>[7x]GGVLVAQDYRAGSFIELLRNRMALAGVGVRILQGLTGNVDIPKRTGASTMYFVDEDVDVTESDGAFGLVGMTPHTAGVATAITRRMMQQGSPDIEALVRDDLLTSLTLGLDKTALVGHSSPSAPNGVRDLVIGDALPFTGPFATFEELVDLETAVASANADVDSMAYIYNAATSGHFKKTLEFAGVSGTIERGGQVNGYNRVKSNQITTAGEVAFGNWSDVVIGMWSGLDLRVDTSTKAASDGKVLRVFTDIDVALRNVESIKWGVPA

We recently characterized a novel roseophage, vB_DshS-R4C (R4C), that could infect the Dinoroseobacter shibae DFL12T, a ubiquitous group of Gram-negative α-proteobacteria of the Roseobacter clade. Here, we report the atomic capsid and in-situ structures of the tail machine of the marine siphophage, vB_DshS-R4C (R4C), which infects Roseobacter. The R4C virion, comprising 12 distinct structural protein components, has a unique five-fold vertex of the icosahedral capsid that allows genome delivery. In this study, we use cryo-electron microscopy (cryo-EM) and structure prediction to determine the atomic structure of the phage R4C capsid and the in-situ structure of the tail machinery to characterize the distinguished long rigid tail.

Using these data, we sought to determine the cryo-EM structure of the R4C capsid head, resolved to an overall resolution of 3.63 Å by cryo-EM single-particle analysis. The R4C capsid shell exhibits a T = 7 quasi-icosahedral lattice with a largest diameter of ~664 Å. The capsid comprises 415 copies of the MCP (vBDshSR4C_006), organized into 11 penton vertexes and 60 hexons. The atomic models of the MCPs within one asymmetric unit containing one hexon plus one pentameric monomer were then built. Through structural superimposition, we find that the overall structure of the R4C MCP is highly similar to HK97 gp5 despite a low sequence identity. Similar to the canonical HK97-fold, the R4C MCP is composed of a long N-terminal arm (N-arm), an axis domain (A-domain), a periphery domain (P-domain), and an extended loop (E-loop). Superimposition of six copies of the hexameric MCP monomer shows conformational heterogeneity, with structural variations primarily located on the E-loop and the N-arm, which contributes to accommodate the deferent radius at deferent location of the capsid shell. A hierarchical network of penton-hexon and hexon-hexon interactions mediate the assembly of the R4C capsid. The penton-hexon interactions are mediated primarily by the two anti-parallel N-arms from neighbouring capsomers; these types of interactions are also observed in hexon-hexon interactions. Unlike the covalently cross-linked chain present in the capsid of HK9737, or the formation of an additional (decoration) protein to stabilize the capsid shells found in phage BPP-141, TW140 and Mic38, the R4C capsid is assembled by non-covalent, inter-capsomeric interactions without any additional decoration.> GSHMDEGKITVFAAASLTNAMQDIATQFKKEKGVDVVSSF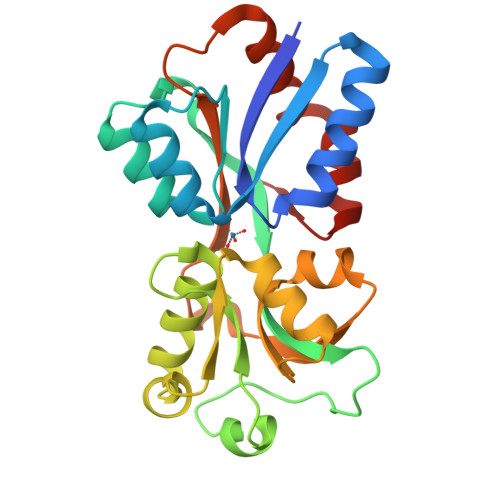ASSSTLARQIEAGAPADLFISADQKWMDYAVDKKAIDTATRQTLLGNSLVVVAPKASVQKDFTIDSKTNWTSLLNGGRLAVGDPEHVPAGIYAKEALQKLGAWDTLSPKLAPAEDVRGALALVERNEAPLGIVYGSDAVASKGVKVVATFPEDSHKKVEYPVAVVEGHNNATVKAFYDYLKGPQAAEIFKRYGFTIK> IVGGQECKDGECPWQALLINEENEGFCGGTILSEFYILTAAHCLYQAKRFKVRVGDRNTEQEEGGEAVHEVEVVIKHNRFTKETYDFDIAVLRLKTPITFRMNVAPACLPERDWAESTLMTQKTGIVSGFGRTHEKGEQSTRLKMLEVPYVDRNSCKLSSSFIITQNMFC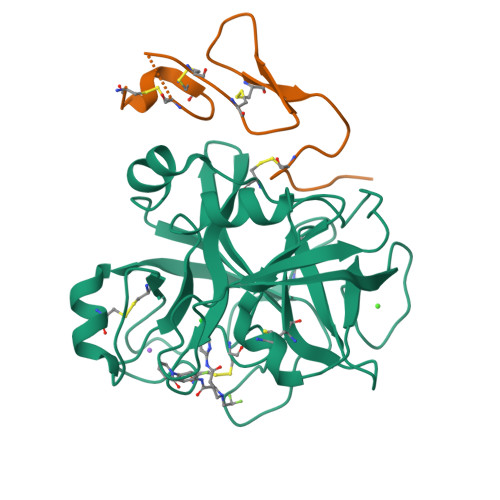AGYDTKQEDACQGDSGGPHVTRFKDTYFVTGIVSWGEGCARKGKYGIYTKVTAFLKWIDRSMKTRGLPKAK;> RKLCSLDNGDCDQFCHEEQNSVVCSCARGYTLADNGKACIPTGPYPCGKQTLERR> MPTQKELRDTMSKKLQEAIKHPDPAVVAGRKSAIKRWVGVLQDNFMEHIKYFKGDKLKFLHNVFQDEGCWSGVRLDNAALGQRFTEEKIGGIDNPLRKYEMACSYCVVDKIHPLFQKRFESYRNKFPPGAFDGKTETEFGKYVRNSLLDSIKRKGPVFDFWIDRESGELKKYDAVEGFDSAVKFKWSEGVEYFYNHLKEEDKEKKLTEAILALSRVQSVEKDAPILDFCVNKIVDKDTLLQKLSQKDKGVYSLFAELIESCFFDTVHDLVQCWCYKEVSAGGDHSEKIFSQRDYELFLSSLSDTMLKNPELSVQARSLIMEFWECGSLYQYRKAAVNTSNYTVPTSGVFAELIVNWRREDIYKTDEEKE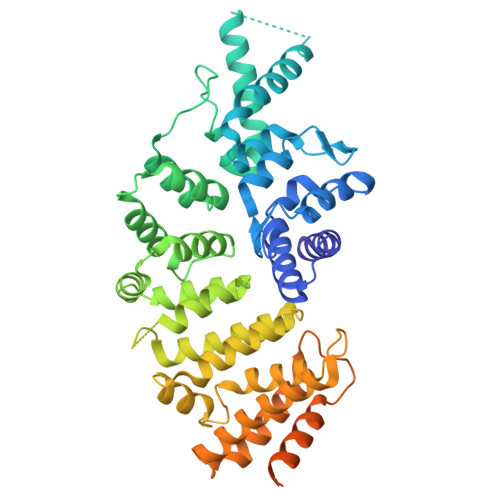IEKKEILDMMSFAKDCFPEKFELFKKLIIRDLRLCGREGKRVNVDYGLFAEELFSELEKTILPPGPVGDGPCSNLRSRSKAHGSKKTTLPVDDSPQSELGTPSVSGVSSYKKKSVFTLSGNKLEHHHHHH> MNDRADFVVPDITTRKN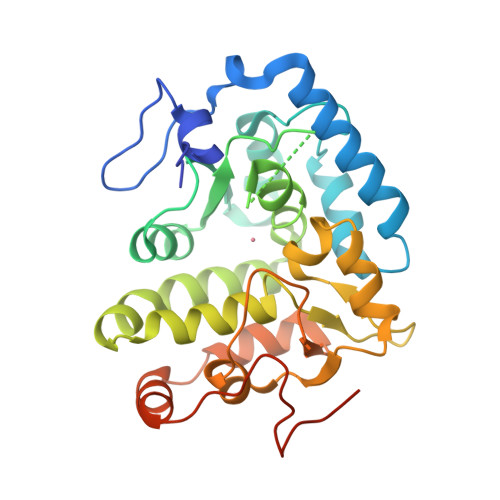VGLSHDANDFTLPQPLDRYSAEDHATWATLYQRQCKLLPGRACDEFLEGLERLEVDADRVPDFNKLNEKLMAATGWKIVAVPGLIPDDVFFEHLANRRFPVTWWLREPHQLDYLQEPDVFHKLFGHVPLLINPVFADYLEAYGKGGVKAKALGALPMLARLYWYTVEFGLINTPAGMRIYGAGILSSKSESIYCLDSASPNRVGFDLMRIMNTRYRIDTFQKTYFVIDSFKQLFDATAPDFAPLYLQLADAQPWGAGDIAPDDLVLNAGDRQGWADTEDV Pgbs are single-domain archaeal heme proteins that are related to the N-terminal domain of globin-coupled sensors (GCSs). In addition to the typical 3-on-3 helical fold found in many globins, the heme group in MaPgb* is completely buried in the protein matrix by a 20-residue N-terminal loop followed by an extra Z-helix and some inter-helical loops with a previously characterized functional role. Thus, the heme is only accessible through two orthogonal tunnels located at the B/G and B/E interfaces (named tunnel 1 and tunnel 2, respectively). Although MaPgb* assembles into a homodimer in solution, this structure does not result in cooperative CO binding.

The cyanide derivative of the ferric Phe(93)E11Tyr and Phe(145)G8Trp MaPgb* mutants (Phe(93)E11Tyr(III)-cyanide and Phe(145)G8Trp(III)-cyanide, respectively) was crystallized by vapor diffusion techniques (protein concentration ~2.6 mM) under conditions matching those for the ligand-free ferric protein. Similar considerations apply to the conserved dimeric assembly; this assembly is based on the following: a four-helix bundle built by the G- and H-helices, the H’-helix, partly the Z-helix, and the BC and FG hinges. Both ferric MaPgb* mutants have been crystallized in the presence of cyanide, which is clearly visible in the electron density of the Phe(93)E11Tyr mutant as the heme-Fe(III)-coordinated ligand but not for the Phe(145)G8Trp mutant, where the heme-Fe(III) atom appears to be free of a distal ligand. In Phe(93)E11Tyr(III)-cyanide, the ligand is bound to the heme-Fe(III) atom with a coordination bond of 2.41 Å and a Fe-C-N angle of 144.7° (2.50 Å and 134.0° in the second dimer subunit). The coordination bond length for cyanide is slightly longer than expected, likely due to partial photoreduction of the heme-Fe(III). Two hydrogen bonds stabilize the heme-Fe(III)-bound cyanide, its N atom being linked to the Tyr(61)B10 OH (2.63 Å and 2.57 Å in the two subunits), and to the Trp(60)B9 N Ɛ2 atom (2.92 and 3.11 Å in the two subunits). The distal site structure and the cyanide-binding mode observed for the Phe(93)E11Tyr(III)-cyanide complex is closely reminiscent of the ligand-binding mode reported for MaPgb*(III)-cyanide. The Tyr(93)E11 side chain of the mutated residue matches the position of the MaPgb*(III)-cyanide Phe(93)E11 residue, with only a small rotation (approximately 5–8°) away from the heme. Thus, in both MaPgb*(III)-cyanide and Phe(93)E11Tyr(III)-cyanide, the aromatic side chain at topological position E11 rotates approximately 90° relative to the position in MaPgb*(III) to provide room for cyanide to bind to Trp(60)B9. As a result of the new Trp(60)B9 side chain location, tunnel 1 is closed in both MaPgb*(III)-cyanide and Phe(93)E11Tyr(III)-cyanide. The consequences of the Phe(93)E11Tyr mutation are quite small, likely because of the comparable sizes of the Phe and Tyr side chains.

>[2x]MSVEKIPGYTYGETENRAPFNLEDLKLLKEAVMFTAEDEEYIQKAGEVLEDQVEEILDTWYGFVGSHPHLLYYFTSPDGTPNEKYLAAVRKRYSRWILDTSNRSYDQAWLDYQYEIGLRHHRTKKNQTDNVESVPNIGYRYLVAFIYPITATMKPFLARKGHTPEEVEKMYQAWFKATTLQVALWSYPYVKYGDF In humans, there are 13 cytosolic sulfotransferases that catalyze the transfer of a sulfuryl group (SO3) from the donor cofactor 3´-phosphate 5´-phosphosulfate (PAPS) to acceptor substrates, including xenobiotics, fatty acids, neurotransmitters, and steroids. Sulfation of 17β-estradiol (E2) by human estrogen sulfotransferase (SULT1E1) results in loss of binding to the estrogen receptor as well as increased availability for renal excretion, thereby effectively regulating the concentration of E2. To understand the binding and inhibition of estrogen sulfotransferase by BFRs, we obtained crystal structures of SULT1E1 in complex with the product cofactor PAP and three different compounds bound at the active site: the natural substrate (E2), a BFR (TBBPA), and a human BFR metabolite (3-OH-BDE-47) at resolutions of 1.95 Å, 2.0 Å, and 2.05 Å, respectively. SULT1E1 crystallizes with two molecules in the asymmetric unit (designated molecule A and molecule B) representing the proposed physiological dimer.

The crystal structure of human SULT1E1 with PAP and E2 bound to the active site is similar in overall fold and substrate binding as previously determined for the mouse estrogen sulfotransferase. In brief, E2 binds to a mostly buried hydrophobic pocket, with the sulfuryl acceptor hydroxyl of E2 within hydrogen bonding distance to the proposed catalytic base His107 and Lys105, placing it in proper position for catalysis. Also contributing to the positioning are Phe80 and Phe141, which flank the planar faces of the phenolic ring of E2. Phe80 and Phe141 have been suggested to function as a steric gate conferring substrate specificity for the enzyme. The crystal structures of E2 bound to estrogen sulfotransferases (mouse and human) do not reveal such an allosteric site.

>MNSELDYYEKFEEVHGILMYKDFVKYWDNVEAFQARPDDLVIATYPKSGTTWVSEIVYMIYKEGDVEKCKEDVIFNRIPFLECRKENLMNGVKQLDEMNSPRIVKTHLPPELLPASFWEKDCKIIYLCRNAKDVAVSFYYFFLMVAGHPNPGSFPEFVEKFMQGQVPYGSWYKHVKSWWEKGKSPRVLFLFYEDLKEDIRKEVIKLIHFLERKPSEELVDRIIHHTSFQEMKNNPSTNYTTLPDEIMNQKLSPFMRKGITGDWKNHFTEALNEKFDKHYEQQMKESTLKFRTEI[2x]> GMDKSAKAPAITIFDHRGCSRAPKESSAKSGSQDDEMLVKVASTKVTVSEDVAAKKLQEFIGFKEKGLDGSV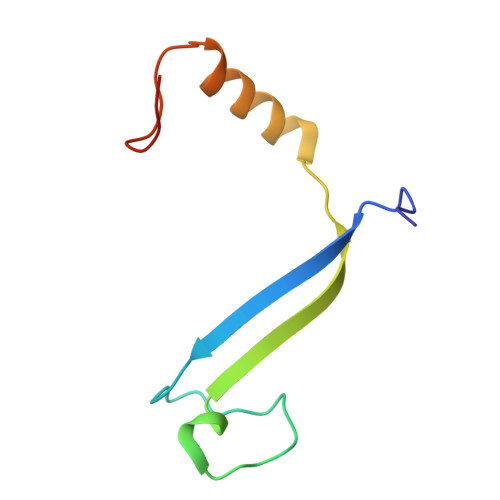IRKK>[5x]STKFSDNYDVKEELGKGAFSVVRRCVHKTTGLEFAAKIINTKKLSARDFQKLEREARICRKLQHPNIVRLHDSIQEESFHYLVFDLVTGGELFEDIVAREFYSEADASHCIQQILESIAYCHSNGIVHRNLKPENLLLASKAKGAAVKLADFGLAIEVNDSEAWHGFAGTPGYLSPEVLKKDPYSKPVDIWACGVILYILLVGYPPFWDEDQHRLYAQIKA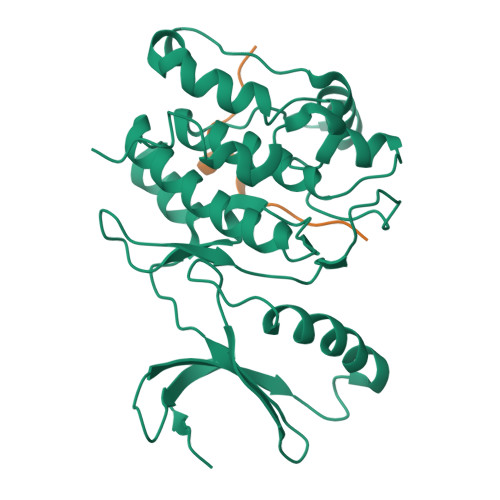GAYDYPSPEWDTVTPEAKSLIDSMLTVNPKKRITADQALKVPWICNRE;>KRPPKLGQIGRSKRVVIA[5x]>GSHMATRDLVLLGEQFREEYKLTQELEMLTDRLQLTLRALEDE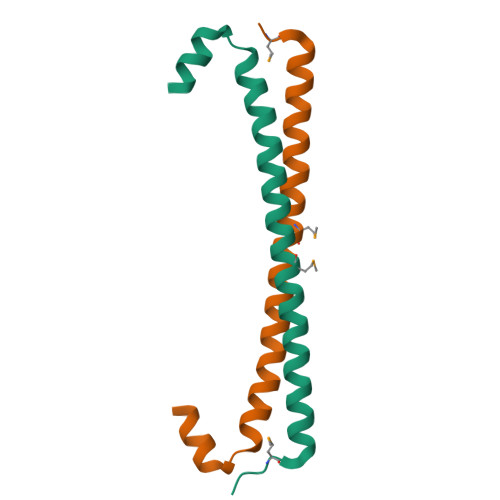KKKTDTLLYSVLPPSVANELRHK[8x]> GSAKDPQAIANRFTSNIKGLTQASRNANDGISIAQTTEGALNEINNNLQRVRELSVQATNGTNSDSDLKSIQDEIQQRLEEIDRVSNQTQFNGVKVLSQDNQMKIQVGANDGETITIDLQKIDVKSLGLDGFNVNGPKEATVGDLKSSFKNVTGYDTYAAGADKYRVDINSGAVVTDAVAPDKVYVNAANGQLTTDDAENNTAVDLFKTTKSTAGTAEAKAIAGAIKGGKEGDTFDYKGVTFTIDTKTGDDGNGKVSTTINGEKVTLTVADIAIGAADVNAATLQSSKNVYTSVVNGQFTFDDKTKNESAKLSDLEANNAVKGESKITVNGAEYTANATGDKITLAGKTMFIDKTASGVSTLINEDAAAAKKSTANPLASIDSALSKVDAVRSSLGAIQNRFDSAITNLGN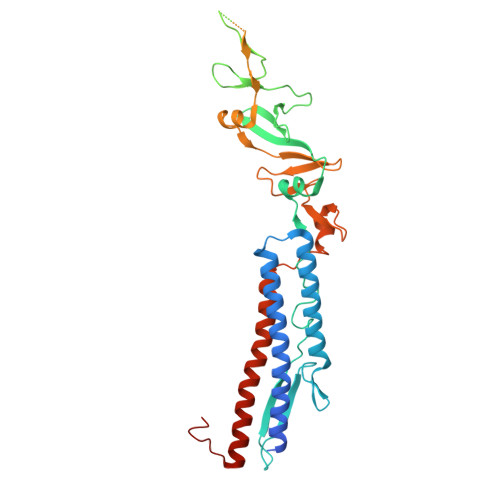TVTNLNSARSRIED>VVKRTMTKKFLEEAFAGESMAHMRYLIFAEKAEQEGFPNIAKLFRAIAYAEFVHAKNHFIALGKLGKTPENLQMGIEGETFEVE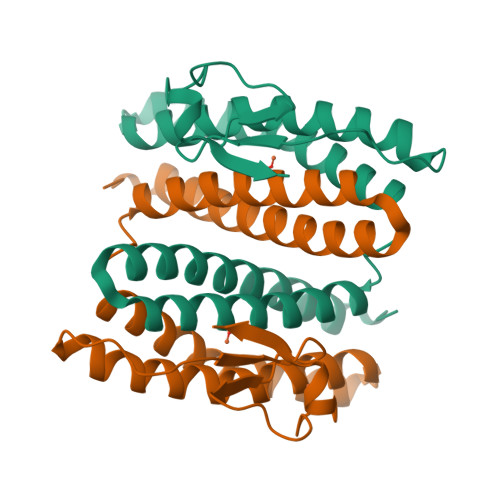EMYPVYNKAAEFQGEKEAVRTTHYALEAEKIHAELYRKAKEKAEKGEDIEIKKVYICPICGYTAVDEAPEYCPVCGAPKEKFVVFE[2x]>[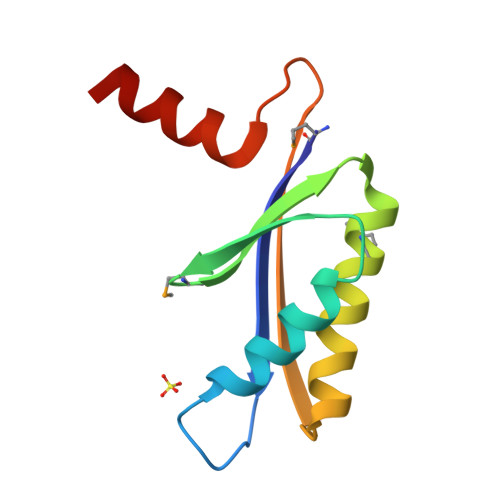4x]MITAELTVIPLGTCSTSLSSYVAAAVEALKKLNVRYEISGMGTLLEAEDLDELMEAVKAAHEAVLQAGSDRVYTTLKIDDRRDADRGLRDKVESVKEKI>MIPGKPWDTPQLAAELERWKLDGRDVSLLIGGPEGLSPACKAAAEQSWSLSALTLPHPLVRVLVAESLYR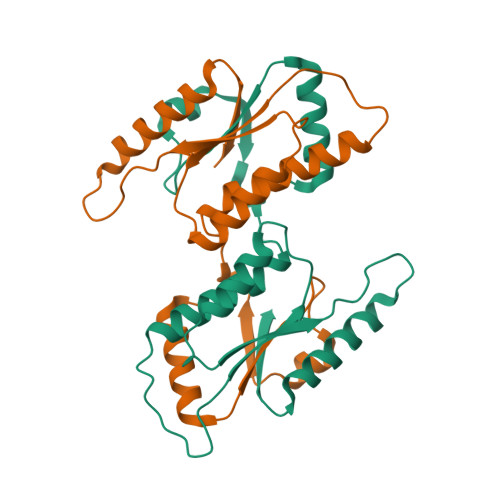AWSITTNHPYHREGSMKLQLVAVGTKMPDWVQTGFTEYLRRFPKDMPFELIEIPAGKRGKNADIKRILDKEGEQMLAAAGKNRIVTLD[4x]>[2x]M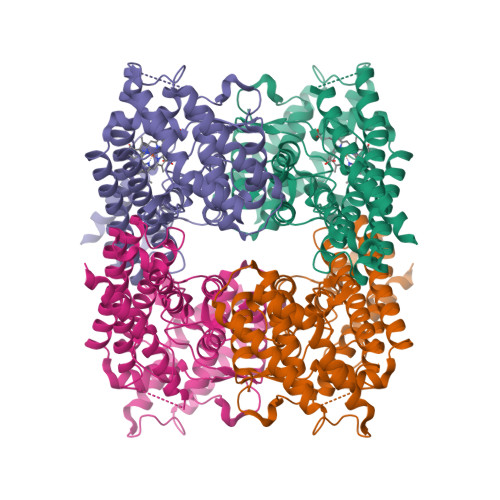KPATYNTEAFDEWIRSRFVELNSQLEQLYYQQTDRANVQEVGTELKHTLESEGRELVKALLDEGNTDEGFDSAFDLLGNVGLYMAACRRHEITEPTRETTSPLLEASALAMHIGASIGVTPRFATAHLTTHNRAHNGIYKRFTDLPDEKLFVDYNTKGILAYKRASDALLKIQPLGISHPISHDLLRVTKQALQDVIESNQQLFNRLDTDRFFYCVRPYYKPYRVGSVVYRGANAGDFAGINVIDLTLGLCFANEASYSQMLVDKFLYMMPEDQQILRECMRRPNLMDDFLQAKGCIHQDWYQENLKLFIEVCELHGQTAIQHHNELVTKYIAEPSVSMEQQHLAKVTASGPPLHVLLASLERLRDRRAAVLRDDIRTRYYDLKKLKDSLRLEHHHHHH>[4x]MKIYVDGREVIINDNERNLLEALKNVGIEIPNLCYLSEASIYGACRMCLVEINGQITTSCTLKPYEGMKVKTNTPEIYEMRRNILELILATHNRDCTTCDRNGSCKLQKYAEDFGIRKIRFEALKKEHVRDESAPVVRDTSKCILCGDCVRVCEEIQGVGVIEFAKRGFESVVTTAFDTPLIETECVLCGQCVAYCPTGALSIRNDIDKLIEALESDKIVIGMIAPAVRAAIQEEFGIDEDVAMAEKLVSFLKTIGFDKVFDVSFGADLVAYEEAHEFYERLKKGERLPQFTSCCPAWVKHAEHTYPQYLQNLSSVKSPQQALGTVIKKIYARKLGVPEEKIFLVSFMPCTAKKFEAEREEHEGIVDIVLTTRELAQLIKMSRIDINRVEPQPFDRPYGVSSQAGLGFGKAGGVFSCVLSVLNEEIGIEKVDVKSPEDGIRVAEVTLKDGTSFKGAVIYGLGKVKKFLEERKDVEIIEVMACNYGCVGGGGQPYPNDSRIREHRAKVLRDTMGIKSLLTPVENLFLMKLYEEDLKDEHTRHEILHTTYRPRRRYPEKDVEILPVPNGEKRTVKVCLGTSCYTKGSYEILKKLVDYVKENDMEGKIEVLGTFCVENCGASPNVIVDDKIIGGATFEKVLEELSKNG;>[4x]MFKNAKEFVQYANKLKTLREKKLNGVSIYVCVGTGCTAKGALKVYSAFEEELKKRNLLGQVTLEKIDDDKVTLNRTGCCGRCSSGPLVKIMPYRFFYSNVAPEDVPEIVDRTVLKGEPIERLFLTDPLTGEKVPRIEDTTLFKNQDFYIMEAIGESECDSIEDYIARSGYESLVKALTSMTPEEIIETVKASGLRGRGGGGFPTGLKWEFTRKAQGDIKFVVCNGDEGDPGAFMNRTLLERDPHLVLEGMIIAGYAVGAQKGYAYIRAEYPFAVKMFKKAIEDARKLGLLGENILGTGFSFDLEVKEGAGAFVCGEETALLASIEGKRGMPRPKPPFPAQSGLWG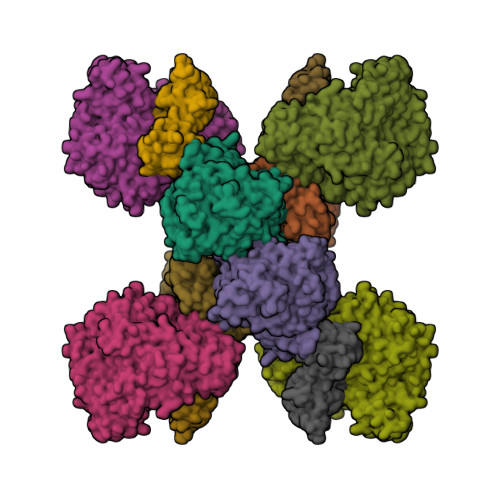KPTLINNVETYANIPRILRDGVENYRKRGTENSPGTKMFSVAGPLKATGIIEVEFGTTLRDIIYNICGGFVEGEEFKAVQIGGPSGACLSEDFIDMPLDYDTLKKADAMVGSGGIVVITKKTCMVEVARFFLDFTKRESCGKCVPCREGTMQAYNILEKFTHGKATYEDLKTLEHLSKTIKTASLCGLGKTAPNPILSTLKLFREEYIAHIEGECPSGMCTAFKKYVINPDICKGCGLCARSCPQNAITGERGKPYTIDQEKCVKCGLCASKCPFKAIELV;>[4x]MASWSHPQFEKSGGGGGENLYFQGAVLALERHFEKVEEILKKYGYKRENLIKILLEIQEIYRYLPEDVINYVSTAMGIPPAKIYGVATFYAQFSLKPKGKYTIMVCDGTACHMAGSPEVLKAIEEETGLTPGNVTEDLMFSLDQVGCLGACALAPVMVINGEVYGNLTADKVKEILRKIKEKERESANV>MVEPMNQSSVFQPPDRQRVDERIATTIADAILDGVFPPGSTLPPERDLAERLGVNRTSLRQGLARLQQMGLIEVRHGSGSKVNNFWETSGLNILETLARLDHESVPQLIDNLLSVRTNISTIFIRTAFRQHPDKAQEVLATANEVADHADAFAELDYNIFRGLAFASGNPIYGLILNGMKGLYTRIGRHYFANPEARSLALGFYHKLSALCSEGAHDQVYETVRRYGHESGEIWHRMQKN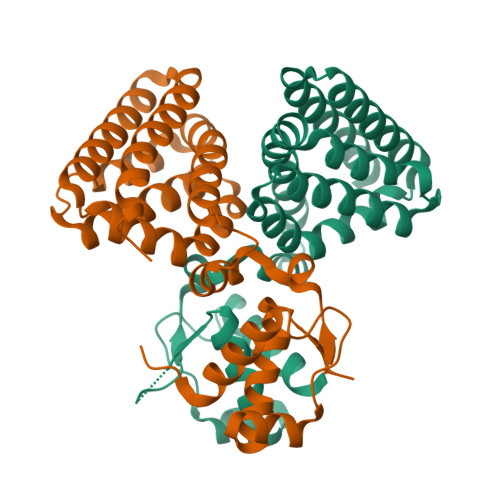LPGDLAIQGR[2x]>GDIIWDQLIVKRTLADLLIPINRQISDIQSTLSEVTTRVHE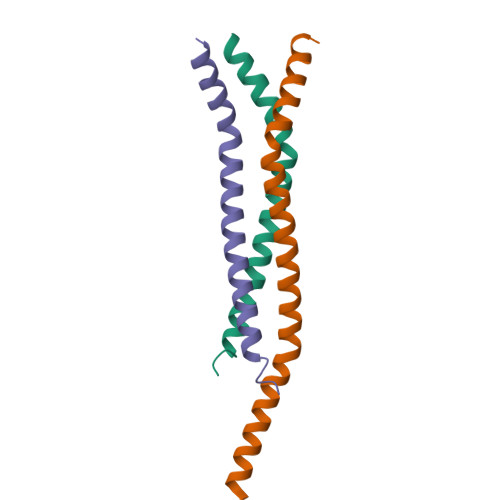IERQLHEITPVLKMGRTLEAISKGMSEMLAK[3x]(1R,2S,3R,5R)-3-(6-amino-9H-purin-9-yl)-5-(hydroxymethyl)cyclopentane-1,2-diol | C11 H15 N5 O3 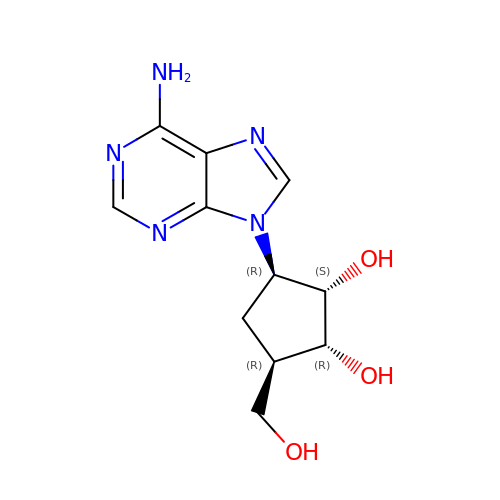| UGRNVLGKAGREKS-GCXDCGAKSA-N> GIDNYEEPSETIWGEVVDEATGKRVLTDQGSEGIRVRLTELSWGDNVQHNPDFYCMMDGTFQNTKIFKGEYNVRIDGPFIPLVRENTDGTLLHDGSVNTEISGTTKVKFEVQPFLNVEFVGNPQVSNGVIKAQVRVTRGVSDEVFREKIQPMGNWKDEYLNVTDIQFFVSYSNTVGYRARDERWSSSINYEGKSFEGLLGKEVTIQSNGNVPSGRKVFV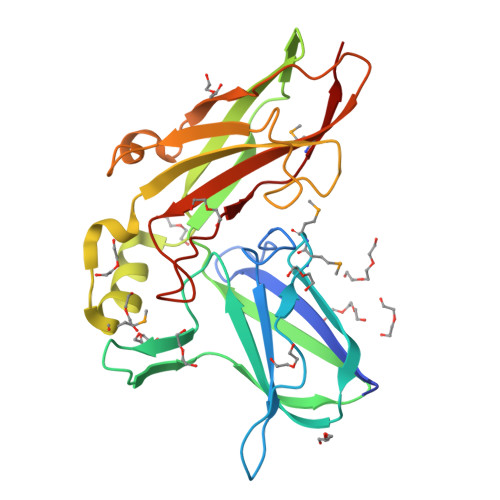RAAARINYDTPVGSGTRRWNYSEPMEVLIP>CGAAXUCG[2x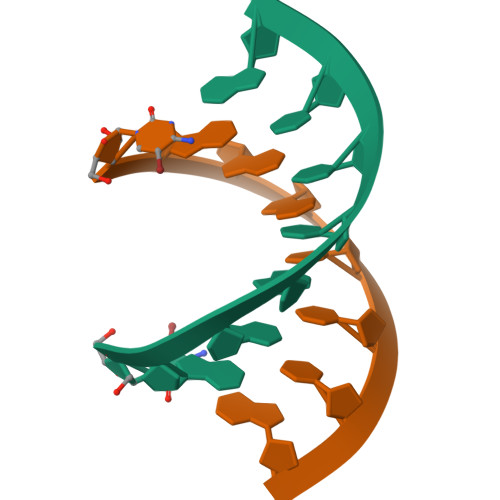]> ITGTSTVGVGRGVLGDQKNINTTYSTYYYLQDNTRGNGIFTYDAKYRTTLPGSLWADADNQFFASYDAPAVDAHYYAGVTYDYYKNVHNRLSYDGNNAAIRSSVHYSQGYNNAFWNGSQMVYGDGDGQTFIPLSGGIDVVAHELTHAVTDYTAGLIYQNESGAINEAISDI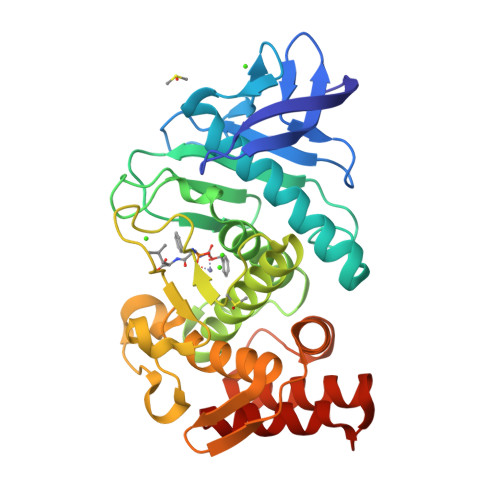FGTLVEFYANKNPDWEIGEDVYTPGISGDSLRSMSDPAKYGDPDHYSKRYTGTQDNGGVHINSGIINKAAYLISQGGTHYGVSVVGIGRDKLGKIFYRALTQYLTPTSNFSQLRAAAVQSATDLYGSTSQEVASVKQAFDAVGVK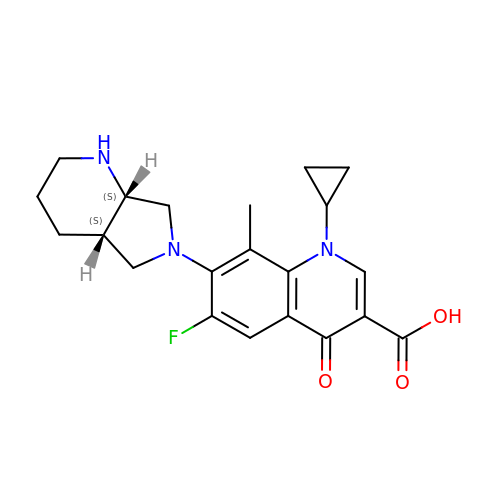1-cyclopropyl-6-fluoro-8-methyl-7-[(4aS,7aS)-octahydro-6H-pyrrolo[3,4-b]pyridin-6-yl]-4-oxo-1,4-dihydroquinoline-3-carboxylic acid | C21 H24 F N3 O3 | LBIDHBYCTAZWKZ-YVEFUNNKSA-N>[2x]DNWRYAHEEYEGDVQDVFAQAFKGYVEDNSDHTVQVYRFGELGESDDIMEQTQNGILQFVNQSPGFTGSLIPSAQIFFIPYLMPTDMDTVLEFFDESKAINEMFPKLYAEHGLELLKMYPEGEMVVTADEPITSPEDFDNKKIRTMTNPLLAETYKAFGATPTPLPWGEVYGGLQTGIIDGQENPIFWIESGG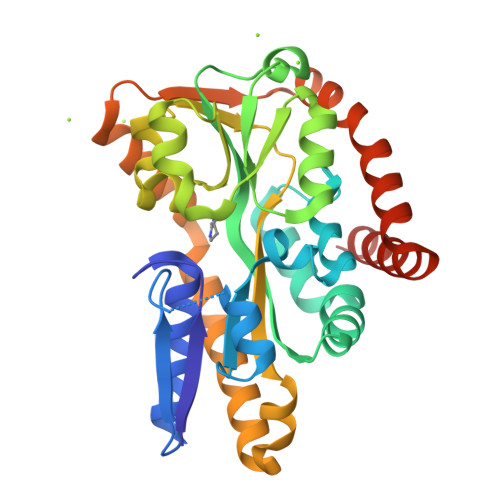LYEVSPNLTFTSHGWFTTAMMANQDFYEGLSEEDQQLVQDAADAAYDHTIEHIKGLSEESLEKIKAASDEVTVTRLNDEQIQAFKERAPQVEEKFIEMTGEQGQELLDQFKADLKAVQSESEG>[2x]IQTTAPPVKESSFVEKMKKTGRNIIVFYGSQTGTAEEFANRLSKDAHRYGMRGMSADPEEYDLADLSSLPEIDKSLVVFCMATYNGDPTDNAQDFYDWLQETDVDLTGVKFAVFGLGNKTYEHFNAMGKYVDQRLEQLGAQRIFELGLGDDDGNLEEDFITWREQFWPAVCEFFGVEATGEESSIRQYELVVHEDMDVAKVYTGEMGRLKSYENQKPPFDAKNPFLAAVTANRKLNQGTERHLMHLELDISDSKIRYESGDHVAVYPANDSALVNQIGEILGADLDVIMSLNNLDEESNKKHPFPCPTTYRTALTYYLDITNPPRTNVLYELAQYASEPSEQEHLHKMA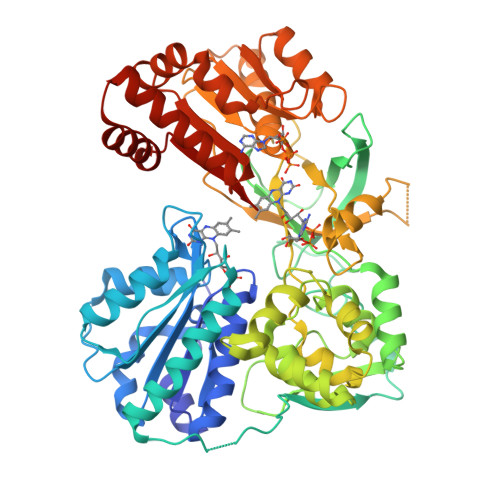SSSGEGKELYLSWVVEARRHILAILQDYPSLRPPIDHLCELLPRLQARYYSIASSSKVHPNSVHICAVAVEYEAKSGRVNKGVATSWLRAKEPAGENGGRALVPMFVRKSQFRLPFKSTTPVIMVGPGTGIAPFMGFIQERAWLREQGKEVGETLLYYGCRRSDEDYLYREELARFHKDGALTQLNVAFSREQAHKVYVQHLLKRDREHLWKLIHEGGAHIYVCGDARNMAKDVQNTFYDIVAEFGPMEHTQAVDYVKKLMTKGRYSLDVWS>[2x]GSFVGSIDQGTTSSRFLIFNGEGNPVASHQIEFENLYPKSGWHEQDPYELLNSVQQCIDGAMHKFASLGYSKENIRAIGITNQRETTVVWDSVTGEPLHNAIVWPDTRTSALVRELKARQSADSLLELCGLPLSTYPSSVKLLWLIQNVDAVKQAYEEGRLAFGTVDSWLIYKLNGGAQAERPIHVTDSTNASRTMFMNLRTLQYDDKLLGFFGIDRNKIKLPKIVPSSDPEAFGKVATGALAGVPIAGCLGDQSSALVGQCGFSPGQAKNTYGTGCFLLYNVGTEPVISKYGLLATVAYDFGRGRKPVYALEGSIAVAGAGITFLMNNLGFAPKPSEINALAESVLDNGGVVFVTAFSGLFAPYWIDDAKGTLFGITQHTTKGHIARATLEATCYQTRAILDAMEKDSGHKLESLAVDGGLSASDLCMQTQADISGIPVDRPRMRETTALGAAIAAGLATGVWRELDHVKESIAGGANGNGKKNAREVFYPKMDRKKAERLFRKWEQAVEMSRGWVREQEEEDGE

Here, we report the first structure of glycerol kinase from the thermophilic filamentous fungus Chaetomium thermophilum (CtGK). Glycerol kinase (EC 2.7.1.30) catalyzes the transfer of phosphate moiety from ATP to glycerol to form glycerol 3-phosphate (G3P). Overall, the CtGK polypeptide chain can be divided into two distinct domains classified by Pfam as FGGY_N (residues 65–325) and FGGY_C (residues 331–583) connected by a flexible region. A similar case is found in CtGK, which forms extended dimers via the interaction between the C-terminal domains with a prominent contribution from hydrophobic residues (Phe422, Gly436, Phe389, Leu394, Thr437, Phe439, Gly440, Ile441, Thr437, Thr445, Leu438, Ile450, Trp580).

We initially determined CtGK in an apo form using ethylene glycol as a cryoprotective agent. The asymmetric unit (ASU) contained two polypeptide chains. The physiological dimer is not contained in the ASU but completed by a symmetry-related chain forming a rather elongated assembly (A:B’ and B:A’). A similar organization was observed for the later structure obtained in P2221 (both chains modeled for the range 65–583 with a gap 541–549). The dimer interaction is mostly mediated by β-strands located on the C-terminal domains. Although crystals were grown from the same condition, the collected datasets were processed in different space groups. We observed that in the absence of nucleotide, CtGK adopts open conformation, which upon nucleotide binding closes up.>MSFVDHPPDWLEEVGEGLREFLGLEAGPPKPKPNQQHQDQARGLVLPGYNYLGPGNGLDRGEPVNRADEVAREHDISYNEQLEAGDNPYLKYNHADAEFQEKLADDTSFGGNLGKAVFQAKKRVLEPFGLVEEGAKTAPTGKRIDDHFPKRKKARTEEDSKPSTSSDAEAGPSGSQQLQIPAQPASSLGADTMSAGGGGPLGDNNQGADGVGNASGDWHCDSTWMGDRVVTKSTRTWVLPSYNNHQYREIKSGSVDGSNANAYFGYSTPWGYFDFNRFHSHWSPRDWQRLINNYWGFRPRSLRVKIFNIQVKEVTVQDSTTTIANNLTSTVQVFTDDDYQLPYVVGNGTEGCLPAFPPQVFTLPQYGYATLNRDNTENPTERSSFFCLEYFPSKMLRTGNNFEFTYNFEEVPFHSSFAPSQNLFKLANPLVDQYLYRFVSTNNTGGVQFNKNLAGRYANTYKNWFPGPMGRTQGWNLGSGVNRASVSAFATTNRMELEGASYQVPPQPNGMTNNLQGSNTYALENTMIFNSQPANPGTTATYLEGNMLITSESETQPVNRVAYNVGGQMATNNQSSTTAPATGTYNLQEIVPGSVWMERDVYLQGPIWAKIPETGAHFHPSPAMGGFGLKHPPPMMLIKNTPVPGNITSFSDVPVSSFITQYSTGQVTVEMEWELKKENSKRWNPEIQYTNNYNDPQFVDFAPDST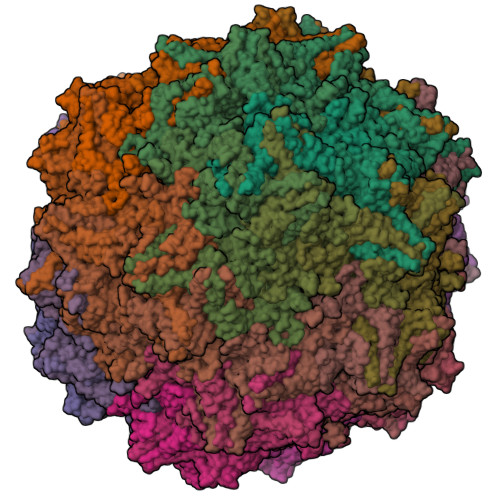GEYRTTRPIGTRYLTRPL[60x]> HKIPAEADFLIAYSTAPGYYSYRNTSNGSWFIQSLCEVLNKYGSELEIMEILTRVNHKVSLRSESSSNDPAFNGKKQMPCFASML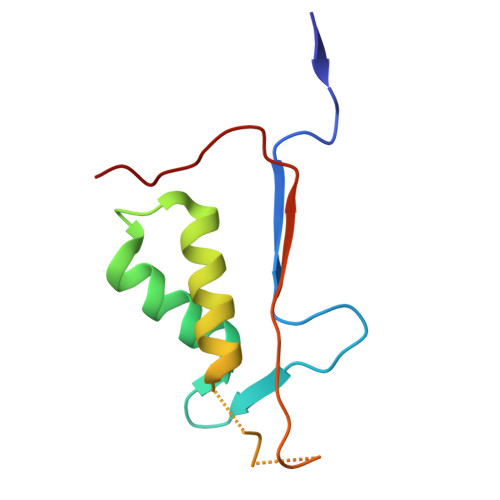TKKLYFSP 (3S,5S,9R,21S)-1-[(2R,3S,4R,5R)-5-(6-amino-9H-purin-9-yl)-4-hydroxy-3-(phosphonooxy)tetrahydrofuran-2-yl]-3,5,9,21-tetrahydroxy-8,8,21-trimethyl-10,14-dioxo-19-thioxo-2,4,6-trioxa-18-thia-11,15-diaza-3,5-diphosphatricosan-23-oic acid 3,5-dioxide | C27 H44 N7 O19 P3 S2 | 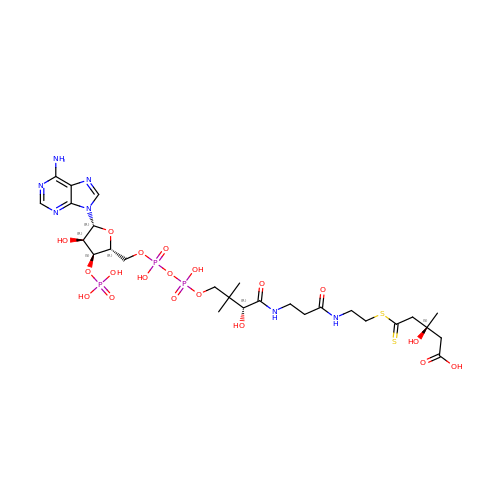JVXXLGZQKQFEOB-VRHQGPGLSA-N>[2x]MKIEPITGSEAEAFHRMGSRAFERYNEFVDLLVGAGIADGQTVVDLCCGSGELEIILTSRFPSLNLVGVDLSEDMVRIARDYAAEQGKELEFRHGDAQSPAGMEDLLGKADLVVSRHAFHRLTRLPAGFDTMLRLVKPGGAILNVSFLHLSDFDEPGFRTWVRFLKERPWDAEMQVAWALAHYYAPRLQDYRDALAQAADETPVSEQRIWVDDQGYGVATVKCFARRAAA

In nature, CouO and NovO catalyze one of the final steps in the biosyntheses of the antibiotics coumermycin A1 and novobiocin, i.e. the methylation of the C-8 atom of the coumarin moiety. Here, we present the high-resolution crystal structure of the C-methyltransferase CouO from Streptomyces rishiriensis in complex with SAH. The overall CouO structure exhibits a core with a Rossmann-like α/β-fold typical of class I SAM-dependent methyltransferases and a cap-domain accommodating two α-helices. Based on this structure and in combination with molecular docking studies and site-directed mutagenesis we identified key functional residues for enzymatic activity and propose an alternative catalytic mechanism for this group of enzymes.

After extensive rebuilding and refinement, two CouO molecules in the asymmetric unit could be completely modeled into the residual electron density. In addition, one SAH cofactor molecule was present in each chain. An analysis of protein-protein interfaces between the two CouO chains in the asymmetric unit using the PDBePISA server identified a dimer interface that is formed by the α-helices of the cap-domain and mainly involves hydrophobic interactions. In CouO, this motif is also present and involves Asp70 forming bidentate interactions with both hydroxyl groups of the ribose. The N-terminal tail of the protein, which is not part of the canonical Rossmann-fold, wraps around the bound cofactor and the side chain of Glu4 forms hydrogen bonds with the amino group of the adenine moiety of SAM/SAH. In this conformation of the N-terminal loop the cofactor would not be able to enter the cavity, indicating and necessitating an increased flexibility of this region upon binding/release of the cofactor. Structure examination of CouO located a cavity in the vicinity of the SAH binding site. Hydrophobic residues are arranged along the central part of the cavity, directly above the sulfur atom of SAH, whereas His and Arg residues are situated on the periphery. The lowest energy docking mode places the coumarin moiety in the vicinity of the cofactor, whereas His120 and Arg121 are situated about 3 Å from the hydroxyl-oxygen at C-7 of the substrate. With His120 playing the role of a general base, the positively charged Arg121 would stabilize the negatively charged intermediate.> MSQQENPKYLWWNHRIIPWEEATVHLTDYWWASVTAVFEVISGYWNNAEGEMYIFRLEDHARRLEQSMQLIRMPKEFTVDEICQATIDLVRANDYRGDVFIMPLAYAVGNKAFSVVGDRTTEMFIYSRPAVSRLEEDFSLHACYSSWTRINERVLPPRIKALANYRNSQLASSEAAMNGYDTALFLNPEGKVAEGTGSCVFFVRKGKLITPDIT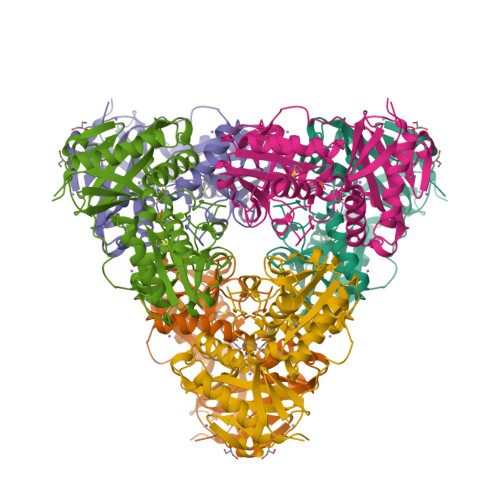SGILESITRDTVIHLAREVLGLEVEERVVDRTETYLADEAFLCGTHAEITPIASIDRHEMKHGAPGPITRQLRDIYREVVYGRDFRYRNWLTPVGMGVRAEQ>MYRDRVRLPSLLDKVMSAAEAADLIQDGMTVGMSGFTRAGEAKAVPQALAMRAKERPLRISLMTGASLGNDLDKQLTEAGVLARRMPFQVDSTLRKAINAGEVMFIDQHLSETVEQLRNHQLKLPDIAVIEAAAITEQGHIVPTTSVGNSASFAIFAKQVIVEINLAHSTNLEGLHDIYIPTYRPTRTPIPLTRVDDRIGSTAIPIPPEKIVAIVINDQPDSPSTVLPPDGETQAIANHLIDFFKREVDAGRMSNSLGPLQAGIGSIANAVMCGLIESPFENLTMYSEVLQDSTFDLIDAGKLRFASGSSITLS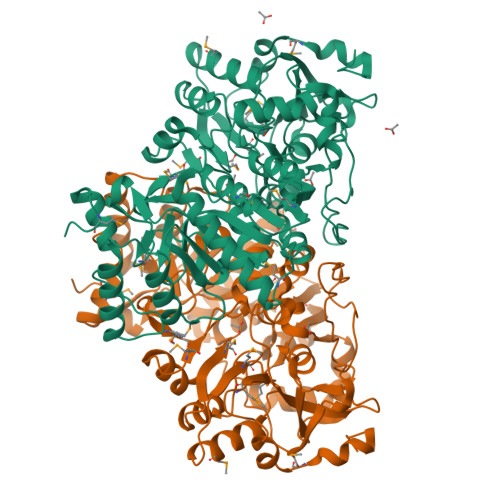PRRNADVFGNLERYKDKLVLRPQEISNHPEVVRRLGIIGINTALEFDIYGNVNSTHVGGTKMMNGIGGSGDFARNAHLAIFVTKSIAKGGNISSVVPMVSHVDHTEHDVDILVTEQGLADLRGLAPRERARVIIENCVHPSYQAPLLDYFEAACAKGGHTPHLLREALAWHLNLEERGHMLAG[2x]>ETGCPANCLCSKTDINCKKPDDGNLFPLLEGQDSGSSNGQTSIQITDISRNITSIHIENWKNLQTLNAVDMELYTGLQRLTIRNSGLRNIQPRAFAKNPHLRYIDLSGNRLTTLSWQLFQTLRLFDLRLERNPFQCSCDIRWIQLWQEKGEANLQSQQLHCMNLDTAVILLRNMNITQCDLPEISVSHVNLTVREGENAVITCQGSGSPLPDVDWTVADLHSINTHQTNLQWTNVHAIQLTLVNVTSEDNGFLLTCIAENVVGMSQASVLLTVYGTKHHHHHH[3x];>ETGESPPVFIKKPVDQIGVSGGVASFVCQATGDPKPRVTWNKKGKKVNSQRFETIEFDESAGAVLRIQPLRTPRDENIYECVAQNPHGEVTVHAKLTVLREDQLPPGFPNIDMGPQLKVVERTRTATMLCAASGNPDPEITWFKDFLPVDPSTSNGRIKQLRSGGLQIESSEETDQGKYECVASNSAGVRYSSPANLYVRVRRVAPRFSILPVSHEIMPGGNVNITCVAVGSPMPYVKWMQGAEDLTPEDDMPVGRNVLELTDVKDSANYTCVAMSSLGVIEAVAQITVKSKGHHHHHH[3x]

At the axonal surface, type IIa receptor protein tyrosine phosphatases (RPTPs) (type IIa RPTPs, for example, RPTPσ, RPTPδ and leukocyte common antigen-related (LAR) in vertebrates, dLAR in Drosophila), are a recently identified nexus for extracellular interactions, receiving signals and transmitting them intracellularly to the cytoskeleton to regulate neuronal extension and guidance, as well as synaptic organization. There are two major neuronal RPTPσ isoforms, sharing a common intracellular catalytic region and an extracellular region predicted to contain three immunoglobulin (Ig)-like domains followed by either five or nine fibronectin (FN) type III domains, in the central and peripheral nervous systems, respectively. Previous mutagenesis and structural studies have demonstrated that the proteoglycan-binding site lies on Ig1 of RPTPσ, and comprises an extended positively charged surface of basic residues101314. Binding of postsynaptic TrkC, is reported to require the N-terminal three Ig domains of RPTPσ17; the NGL-3-binding site has been mapped to the FN1-2 domains.

We had noted that the interaction affinity between engineered proteins used for RPTPσ:TrkC complex crystallization (chicken RPTPσ Ig1–3 and TrkC LRRIg1cryst) was some 20-fold lower following the TrkC 63–77 loop deletion (Kd 4.8 μM versus 216 nM). We therefore explored the possible contribution of the 63–77 loop to the RPTPσ:TrkC interaction by engineering a construct termed TrkC LRRIg12Q, comprising the full sequence but still removing two predicted N-linked glycosylation sites by introducing N68Q and N72Q mutations. This construct did indeed bind RPTPσ with enhanced affinity, while TrkC TM2Q induced comparable levels of presynaptic differentiation in co-cultured rat hippocampal neurons to wild-type TrkC TM. We determined the 3.05 Å crystal structure of this chicken RPTPσ Ig1–3:TrkC LRRIg12Q complex in an attempt to visualize this additional, fourth, binding site. Crystals grew in a new space group, P1, with three RPTPσ:TrkC complexes in the asymmetric unit (a.s.u.). The site 4 interface is not well resolved in this 3.05-Å resolution structure, although we do observe an additional TrkC helix (formed by residues 69–80), which interacts with RPTPσ Ig2 predominantly via potential packing of the I73 side chain against a hydrophobic region consisting of RPTPσ residues V144, Y223 and TrkC L56, T74 and L101. The RPTPσ Ig2–Ig3 linker (V226-A230) and the Ig3 domain also lack well-ordered electron density in this structure. However, a R227A+R228A double mutation reduced RPTPσ:TrkC binding, as did insertion of the meB mini-exon between R225 and V226 in SPR-binding assays, supporting the involvement of the RPTPσ Ig2–Ig3 linker in the auxilary binding site 4.> SMEDRAAQSLLNKLIRSNLVDNTNQVEVLQRDPNSPLYSVKSFEELRLKPQLLQGVYAMGFNRPSKIQENALPLMLAEPPQNLIAQSQSGTGKTAAFVLAMLSQVEPANKYPQCLCLSPTYELALQTGKVIEQMGKFYPELKLAYAVRGNKLERGQKISEQIVIGTPGTVLDWCSKLKFI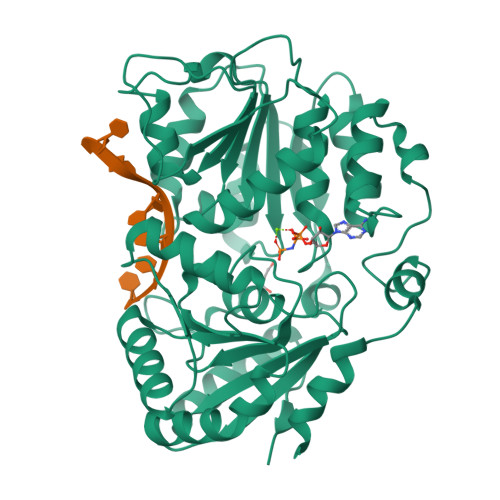DPKKIKVFVLDEADVMIATQGHQDQSIRIQRMLPRNCQMLLFSATFEDSVWKFAQKVVPDPNVIKLKREEETLDTIKQYYVLCSSRDEKFQALCNLYGAITIAQAMIFCHTRKTASWLAAELSKEGHQVALLSGEMMVEQRAAVIERFREGKEKVLVTTNVCARGIDVEQVSVVINFDLPVDKDGNPDNETYLHRIGRTGRFGKRGLAVNMVDSKHSMNILNRIQEHFNKKIERLDTDDLDEIE> MTSQKLVRLPGLIDVHVHLREPGGTHKEDFASGTAAALAGGITMVCAMPNTRPPIIDAPALALAQKLAEAGARCDFALFLGASSENAGTLGTVAGSAAGLALYLNETFSELRLDSVVQWMEHFETWPSH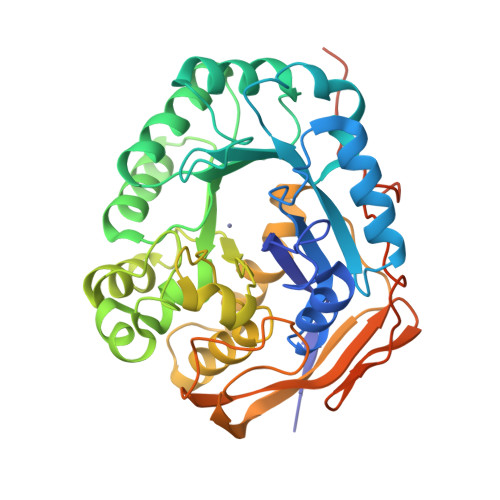LPIVAHAEQQTVAAVLMVAQLTQRSVHICHVARKEEILLIKAAKARGLPVTCEVAPHHLFLSHDDLERLGPGKGEVRPELGSRQDVEALWENMAVIDCFASDHAPHTLEEKCGSRPPPGFPGLETMLPLLLTAVSEGRLSLDDLLQRLHHNPRRIFHLPPQEDTYVEVDLEHEWTIPSHMPFSKAHWTPFEGQKVKGTVRRVVLRGEVAYIDGQVLVPPGYGQDVRKWPQGAVPQLPPSAPATSEMTTTPERPRRGIPGLPD> CDIHVLWEWK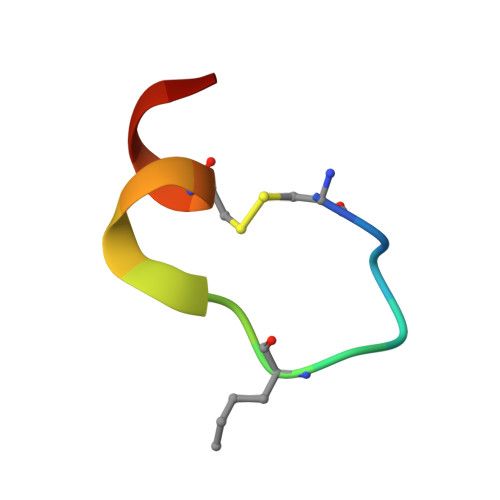CFEEL>SLKKIVESTTFPRTKQSITEDLKALGLKKGMTVLVHSSLSSIGWVNGGAVAVIQALIDVVTEEGTIVMPSQSVELSDPKEWGNPPVPEEWWDIIRESMPAYNSNYTPTTRGMGQIVELFRSYPEVKRSNHPNYSFVAWGKHKNKILNQHPLEFGLGEQSPLGKLYIRESYVLLLGADFDSSTCFHLAEYRIPYQKIINRGAPIIVEGKRVWKEYKELEFREELFQEVGQAFEAEHNMKVGKVGSANCRLFSLTEAVDFAE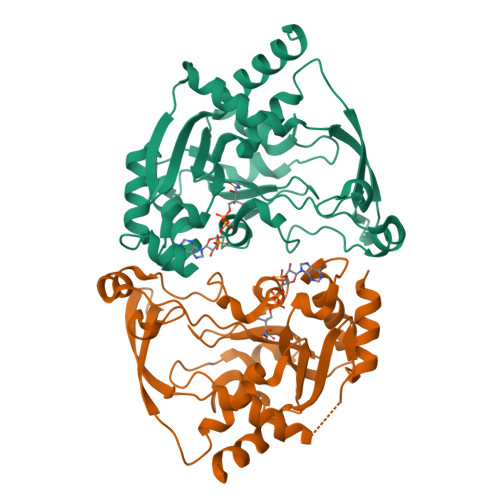KWFINNDSKNIKK[6x]>MTSTVEFINRWQRIALLSQSLLELAQRGEWDLLLQQEVSYLQSIETVMEKQTPPGITRSIQDMVAGYIKQTLDNEQLLKGLLQQRLDELSSLIGQSTRQKSLNNAYGRLSG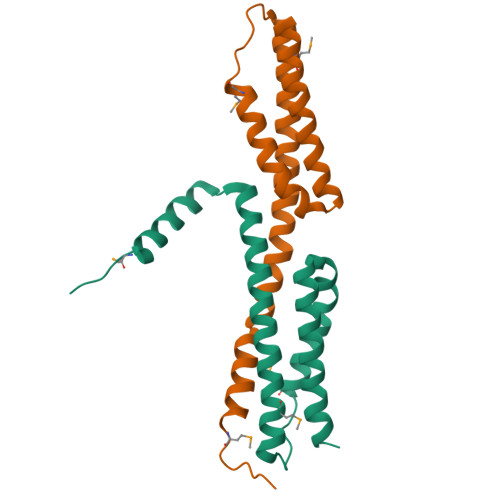MLLVPDAPGAS[2x]>MKVLVTGFEPFGGEKINPTERIAKDLDGIKIGDAQVFGRVLPVVFGKAKEVLEKTLEEIKPDIAIHVGLAPGRSAISIERIAVNAIDARIPDNEGKKIEDEPIVPGAPTAYFSTLPIKKIMKKLHERGIPAYISNSAGLYLSNYVMYLSLHHSATKGY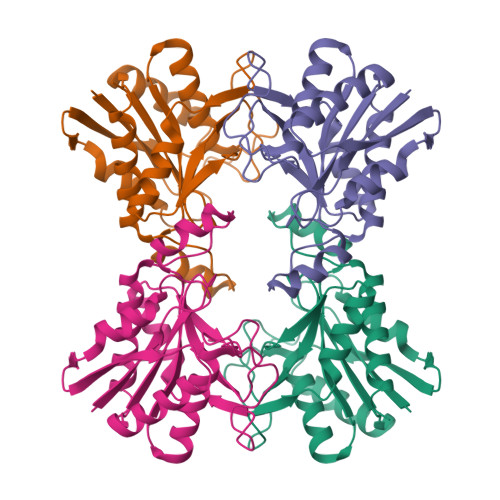PKMSGFIHVPYIPEQIIDKIGKGQVPPSMSYEMELEAVKVAIEVALEELL[4x]>SSLAEKDIQYQLHPYTNARLHQELGPLIIERGQGIYVYDDQGKGYIEAMAGLWSAALGFSNQRLIKAAEQQFNTLPFYHLFDHKSHRPSIELAEKLIEMAPVPMSKVFFTNSGSEANDTVVKMVWYLNNALGKPAKKKFISRVNGYHGVTVASASLTGLPGNQRGFDLPLPGFLHVGCPHHYRFALAGESEEHFADRLAVELEQKILAEGPETIAAFIGEPLMGAGGVIVPPRTYWEKIQKVCRKYDILVIADEVICGFGRTGQMFGSQTFGIQPDIMVLSKQLSSSYQPIAAILINAPVFEGIADQSQALGALGHGFTGSGHPVATAVALENLKIIEEESLVEHAAQMGQLLRSGLQHFIDHPLVGEIRGCGLIAAVELVGDRVSKAPYQALGTL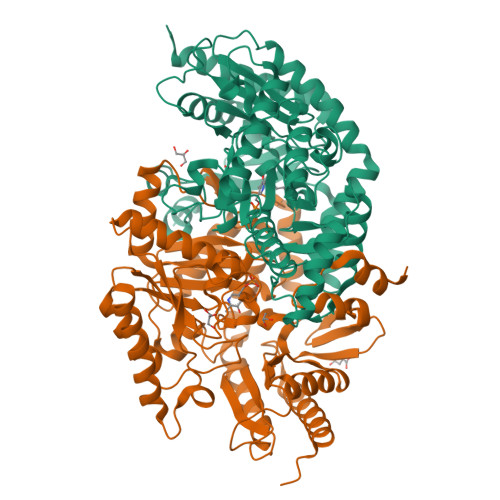GRYMAGRAQEHGMITRAMGDAVAFCPPLIVNEQEVGMIVERFARALDDTTQWVGPGG[2x]> PFLELDTNLPANRVPAGLEKRLCAAAASILGKPADRVNVTVRPGLAMALSGSTEPCAQLSISSIGVVGTAEDNRSHSAHFFEFLTKELALGQDRILIRFAPLESWQIGKIGTVM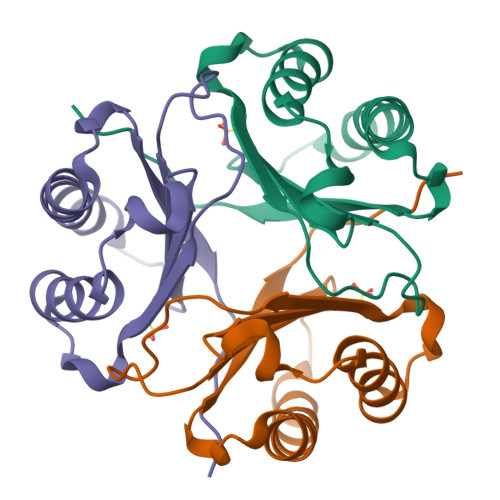TFL> GPGMSTGGDFGNPLRKFKLVFLGEQSVGKTSLITRF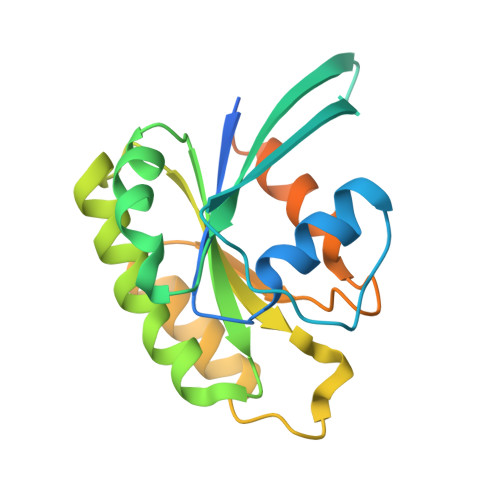MYDSFDNTYQATIGIDFLSKTMYLEDRTVRLQLWDTAGLERFRSLIPSYIRDSTVAVVVYDITNVNSFQQTTKWIDDVRTERGSDVIIMLVGNKTDLADKRQVSIEEGERKAKELNVMFIETSAKAGYNVKQLFRRVAAALPGMESTQDRSREDMIDIKLEKPQEQPVSEGGCLL Two Agrobacterium ABC-transporters and their cognate periplasmic binding proteins (PBPs) OccJ and NocT import octopine and nopaline/octopine, respectively. Recognition and import of opines are conferred by periplasmic binding proteins (PBPs) and their associated ATP-binding cassette (ABC) transporters. The PBP OccJ is associated with the octopine transporter of octopine-type A. tumefaciens while NocT is associated with nopaline uptake in the nopaline-type A. tumefaciens. OccJ shares 47% sequence identity with NocT and belongs to cluster F within the PBP structural classification.

In parallel, we produced the corresponding reciprocal mutant in NocT, in which Gly97 was replaced by a serine. As expected, the presence of the serine at position 97 in NocT abolished the nopaline binding ability whereas octopine binding was preserved but with a 10-fold lower affinity compared with the WT. Therefore, in contrast to OccJ, a serine at position 97 does not favour high affinity for octopine in NocT. We thus validated that the presence of Gly97 in NocT was essential for the spatial accommodation of the α-ketoglutarate moiety of nopaline. We solved the structure of NocT-G97S in complex with octopine at 2.35 Å. Remarkably, both octopine molecules overlap and adopt a similar conformation, unlike observations in OccJ. Therefore, the G97S mutation has a low impact on the protein mutant-octopine interactions compared with the WT, in line with affinity towards octopine in the same range. Moreover, Ser97 exhibits different conformations in both molecules of the asymmetric unit of the NocT-G97S-octopine structure and each of it is not compatible with a bound nopaline. Replacing Gly97 with a serine lead to a selective octopine binding protein by restricting the opine volume. Indeed, the NocT mutant can no longer accommodate nopaline, which is bulkier than octopine.

>MKDYKSITIATEGSYAPYNFKDAGGKLIGFDIDLGNDLCKRMNIECKFVEQAWDGIIPSLTAGRYDAIMAAMSIQPAREKVIAFSRPYLLTPMTFLTTADSPLLKTQVAIENLPLDNITPEQKAELDKFTKIFEGVKFGVQAGTSHEAFMKQMMPSVQISTYDTIDNVVMDLKAGRIDASLASVSFLKPLTDKPDNKDLKMFGPRMTGGLFGKGVGVGIRKEDADLKALFDKAIDAAIADGTVQKLSQQWFGYDASPKQHHHHHH[2x]>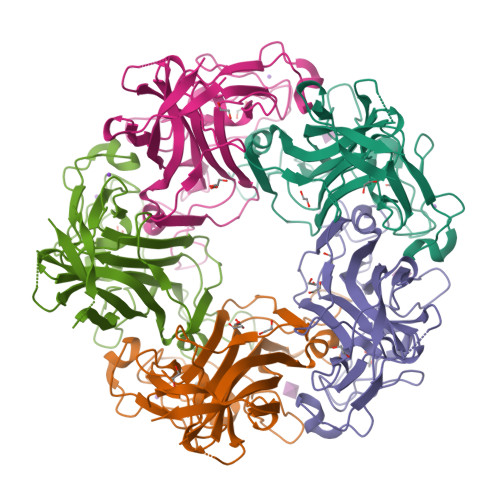[5x]GSHMGGVEVLEVKTGVDSITEVECFLTPEMGDPDEHLRGFSKSISISDTFESDSPNKDMLPCYSVARIPLPNLNEDLTCGNILMWEAVTLKTEVIGVTTLMNVHSNGQATHDNGAAKPVQGTSFHFFSVGGEALELQGVVFNYRTTYPDGTIFPKNATVQSQVMNTEHKAYLDKNKAYPVECWVPDPTRNENTRYFGTLTGGENVPPVLHITNTATTVLLDEFGVGPLCKGDNLYLSAVDVCGMFTNRSGSQQWRGLSRYFKVQLRKRRVKN>[2x]GFQTFEGDLKWHHHNITYWIQNYSEDLPRAVIDDAFARAFALWSAVTPLTFTRVYSRDAD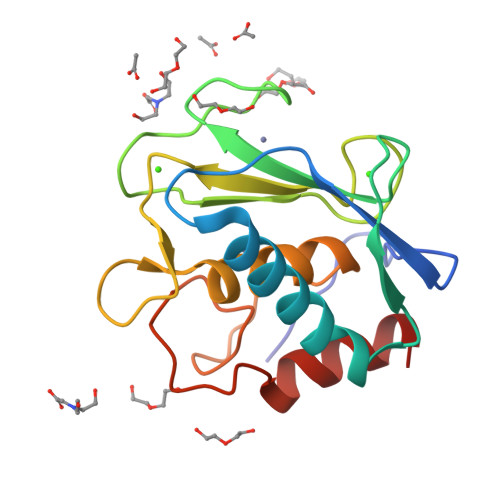IVIQFGVAEHGDGYPFDGKDGLLAHAFPPGPGIQGDAHFDDDELWSLGKGVGYSLFLVAAHEFGHALGLDHSSVPEALMYPMYRFTEGPPLHKDDVNGIRHLYG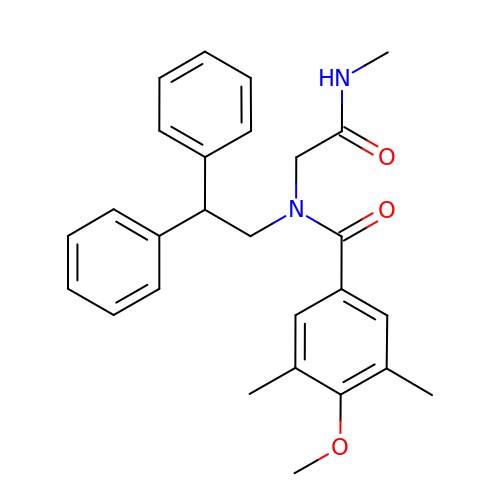N-(2,2-diphenylethyl)-4-methoxy-3,5-dimethyl-N-[2-(methylamino)-2-oxidanylidene-ethyl]benzamide | C27 H30 N2 O3 | NLJFSVIZSWAERX-UHFFFAOYSA-N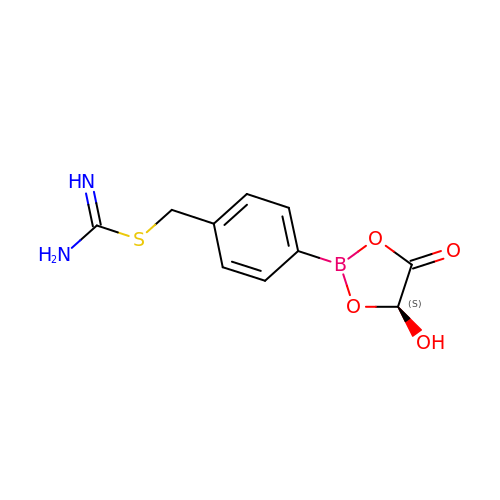[4-[(4~{S})-4-oxidanyl-5-oxidanylidene-1,3,2-dioxaborolan-2-yl]phenyl]methyl carbamimidothioate | C10 H11 B N2 O4 S | OMOMPYVBIXPZLY-QMMMGPOBSA-N7-[4-(aminomethyl)phenyl]-4-methylquinolin-2-amine | C17 H17 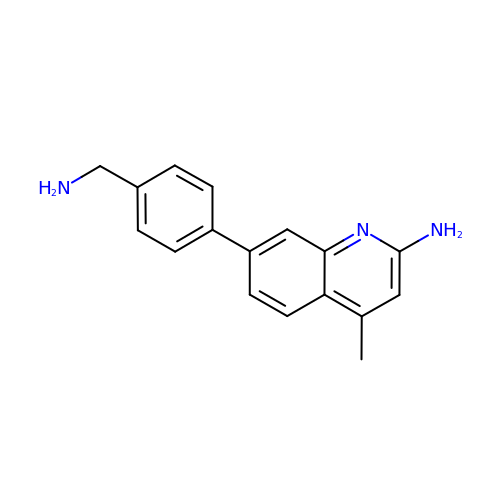N3 | ODOXISOTMVXLOX-UHFFFAOYSA-N>[12x]DSKKIVGVFYKANEYATKNPNFLGCVENALGIR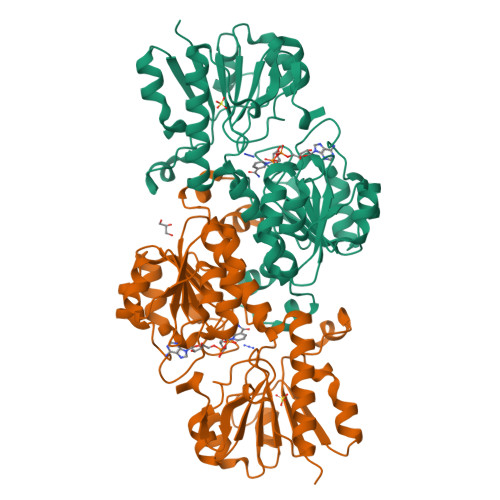DWLESQGHQYIVTDDKEGPDCELEKHIPDLHVLISTPFHPAYVTAERIKKAKNLKLLLTAGIGSDHIDLQAAAAAGLTVAEVTGSNVVSVAEDELMRILILMRNFVPGYNQVVKGEWNVAGIAYRAYDLEGKTIGTVGAGRIGKLLLQRLKPFGCNLLYHDRLQMAPELEKETGAKFVEDLNEMLPKCDVIVINMPLTEKTRGMFNKELIGKLKKGVLIVNNARGAIMERQAVVDAVESGHIGGYSGDVWDPQPAPKDHPWRYMPNQAMTPHTSGTTIDAQLRYAAGTKDMLERYFKGEDFPTENYIVKDGELAPQYR>[5x]GERPRSEEDNELNLPNLAAAYSSILSSLGENPQRQGLLKTPWRAASAMQFFTKGYQETISDVLNDAIFDEDHDEMVIVKD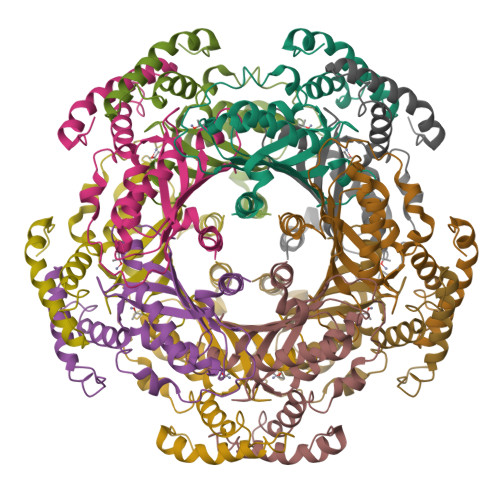IDMFSMCEHHLVPFVGKVHIGYLPNKQVLGLSKLARIVEIYSRRLQVQERLTKQIAVAITEALRPAGVGVVVEATHMCMVMRGVQKMNSKTVTSTMLGVFREDPKTREEFLTLIRS>MMSETAPLPSASSALEDKAASAPVVGIIMGSQSDWETMRHADALLTELEIPHETLIVSAFRTPDRLADYARTAAERGLNVIIAGAGGAAHLPGMCAAWTRLPVLGVPVESRALKGMDSLLSIVQMPGGVPVGTLAIGASGAKNAAL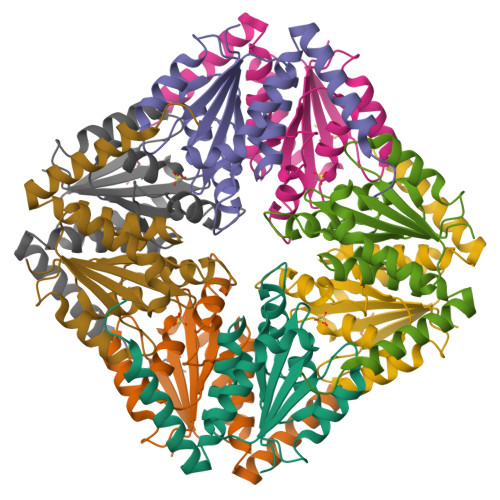LAASILALYNPALAARLETWRALQTASVPNSPITEDK[2x]> GAMGTSLFTDRATNQLYVLLSGQLHPVYNLTSARLVLGNPANPATVKSSELSKLPMGQTVGIPGAPYATPVSAGSTSIWTLCDTVARADSTSPVVQTAVIAMPLEIDASIDPLQSHEAVLVSYQGETWIVTTKGRHAIDLTDRALTSSMGIPVTARPTPISEGMFNALPDMGPWQLPPIPAAGAPNSLGLPDDLVIGSVFQIHTDKGPQYYVVLPDGIAQVNATTAAALRATQAHGLVAPPAMVPSLVVRIAERVYPSPLPDEPLKIVSRPQDPALCWSWQRSAGDQSPQSTVLSGRHLPISPSAMNMGIKQIHGTATVYLDGGKFVALQSPDPRYTESMYYIDPQGVRYGVPNAETAKSLGLSSPQNAPWEIVR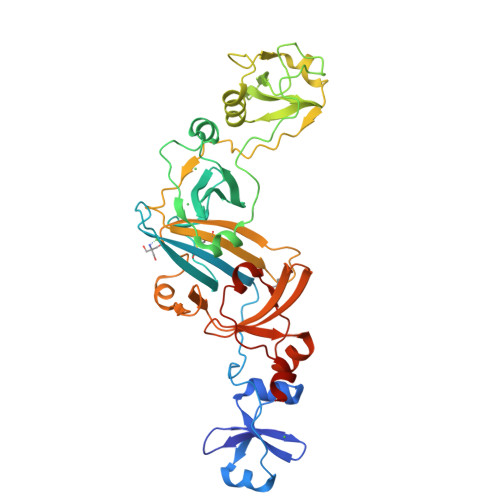LLVDGPVLSKDAALLEHDTL> APDTSVSNKQNFSTDVIYQIFTDRFSDGNPANNPTGAAFDGTCTNLRLYCGGDWQGIINKINDGYLTGMGVTAIWISQPVENIYSIINYSGVNNTAYHGYWARDFKKTNPAYGTIADFQNLIAAAHAKNIKVIIDFAPNHTSPASSDQPSFAENGRLYDNGTLLGGYTNDTQNLFHHNGGTDFSTTENGIYKNLYDLADLNHNNSTVDVYLKDAIKMWLDLGIDGIRMAAVKHMPFGWQKSFMAAVNNYKPVFTFGAWFLGVNEVSPENHKFANESGMSLLDFRFAQKVRQVFRDNTDNMYGLKAMLEGSAADYAQVDDQVTFIDNHDMERFHASNANRRKLEQALAFTLTSRGVPAIYYGTEQYMSGGTDPDNRARIPSFSTSTTAYQVIQKLAPLRKSNPAIAYGSTQERWINNDVLIYERKFGSNVAVVAVNRNLNAPASISGLVTSLPQGSYNDVLGGLLNGNTLSVGSGGAASNFTLAAGGTAVWQYTAATATPTIGHVGPMMAKPG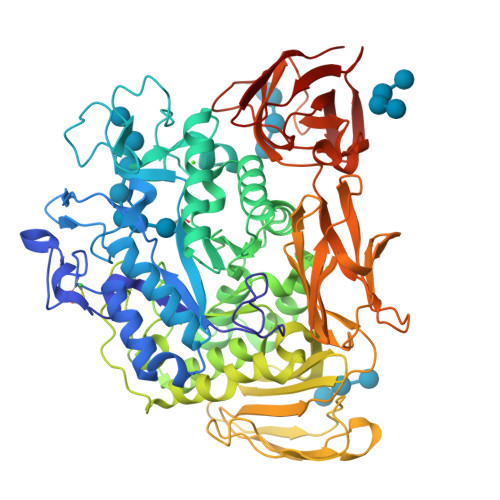VTITIDGRGFGSSKGTVYFGTTAVSGADITSWEDTQIKVKIPAVAGGNYNIKVANAAGTASNVYDNFEVLSGDQVSVRFVVNNATTALGQNVYLTGSVSELGNWDPAKAIGPMYNQVVYQYPNWYYDVSVPAGKTIEFKFLKKQGSTVTWEGGSNHTFTAPSSGTATINVNWQP>MGHHHHHHENLYFQGHMQNVSLRELAEKLNIYIGFAAINNFWSLSDEEKYMEVARREFNILTPENQMKWDTIHPERDRYNFTPAEKHVEFAEENNMIVHGHTLVWHNQLPGWITGREWTKEELLNVLEDHIKTVVSHFKGRVKIWDVVNEAVSDSGTYRESVWYK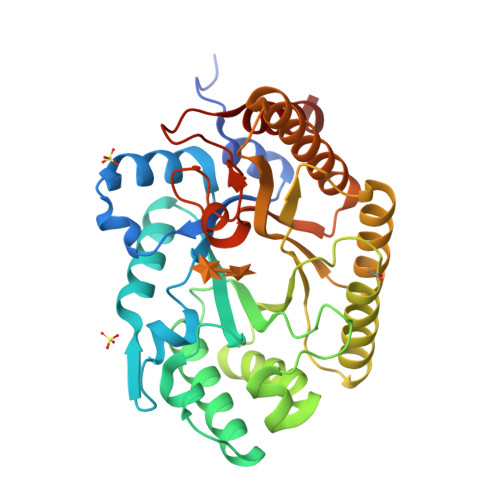TIGPEYIEKAFRWTKEADPDAILIYNDYSIEEINAKSNFVYNMIKELKEKGVPVDGIGFQMHIDYRGLNYDSFRRNLERFAKLGLQIYITEMDVRIPLSGSEDYYLKKQAEICAKIFDICLDNPAVKAIQFWGFTDKYSWVPGFFKGYGKALLFDENYNPKPCYYAIKEVLEKKIE[2x]>[4x]ERSAVQLSLSSRLQLTLYQYKTCPFCSKVRAFLDFHALPYQVVEVNPVLRAEIKFSSYRKVPILVAQEGESSQQLNDSSVIISALKTYLVSGQPLEEIITYYPA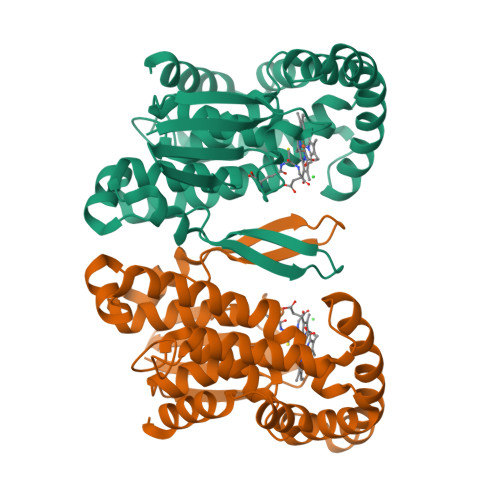MKAVNDQGKEVTEFGNKYWLMLNEKEAQQVYSGKEARTEEMKWRQWADDWLVHLISPNVYRTPTEALASFDYIVREGKFGAVEGAVAKYMGAAAMYLISKRLKSRHRLQDNVREDLYEAADKWVAAVGKDRPFMGGQKPNLADLAVYGVLRVMEGLDAFDDLMQHTHIQPWYLRVERAITEASPAH>[8x]MHCPFCRHPDSRVVDSRTTDDGTSIRRRRQCPDCSRRFTTVETCSLMVVKRSGVTEPFSRTKVINGVRKACQGRPV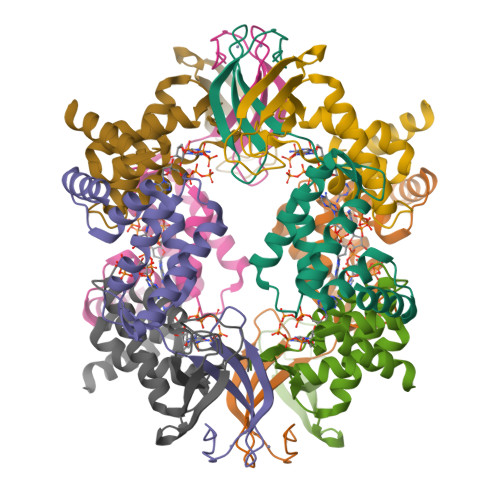TEDALAQLGQRVEEAVRATGSAELTTHDVGLAILGPLQELDLVAYLRFASVYRAFDSLEDFEAAIAELRETTGHPGEEDDTGAGSQENDRGPTGAGQVPEPAGAADKLAAALEHHHHHH IMIDO DIPHOSPHATE | H3 N O6 P2 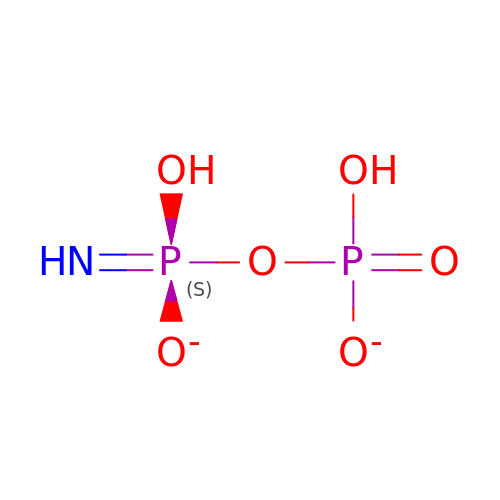| VYBCVOULKDXKCH-UHFFFAOYSA-M>[2x]MKEIPYAELLGILSAQPTWDRSNGFHSVVDQYPEFKMVAQQSAEFDRDTAYKVTEQILQAHPEIKAIWCGNDAMALGAMKACEAAGRTDIYIFGFD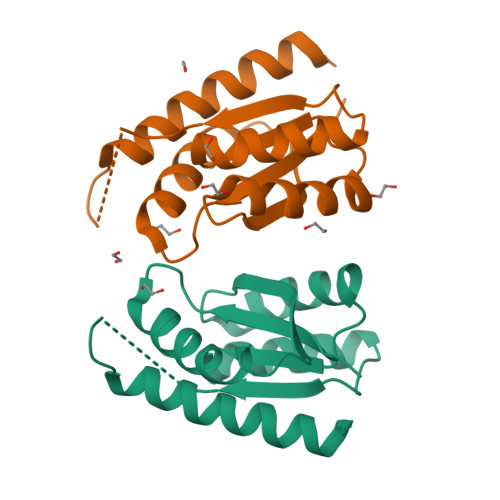GAEDVINAIKEGKQIVATIMVGHNHNYYGGVLAGEYFVKFLKEKYPDGGHHHHHH> VVHGQTAKTITIKVDTFKDRKPISPYIYGTNQDLAGDENMAARRLGGNRMTGYNWENNMSNAGSDWQQSSDNYLCSNGGLTQAECEKPGAVTTSFHDQSLKLGTYSLVTLPMAGYVAKDGNGSVQESEAAPSARWNQVVNAKNAPFQLQPDLNDNYVYVDEFV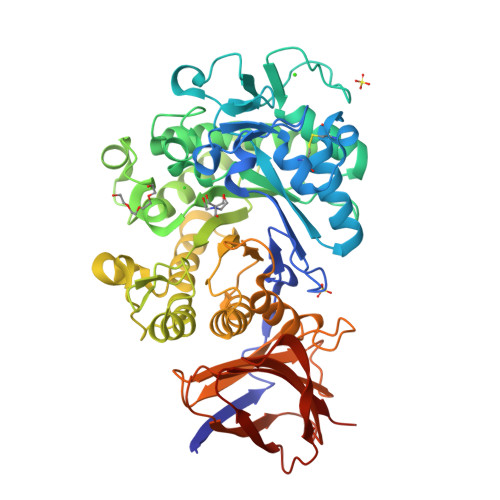HFLVNKYGTASTKAGVKGYALDNEPALWSHTHPRIHGEKVGAKELVDRSVSLSKAVKAIDAGAEVFGPVLYGFGAYKDLQTAPDWDSVKGNYSWFVDYYLDQMRLSSQVEGKRLLDVFDVHWYPEAMGGGIRITNEVGNDETKKARMQAPRTLWDPTYKEDSWIAQWNSEFLPILPRLKQSVDKYYPGTKLAMTEYSYGGENDISGGIAMTDVLGILGKNDVYMANYWKLKDGVNNYVSAAYKLYRNYDGKNSTFGDTSVSAQTSDIVNSSVHASVTNASDKELHLVVMNKSMDSAFDAQFDLSGAKTYISGKVWGFDKNSSQIKEAAPITQISGNRFTYTVPPLTAYHIVLTTGNDTSPV>[3x]ATVGPRVIVVGAGMSGISAAKRLSEAGITDLLILEATDHIGGRMHKTNFAGINVELGANWVEGVNGGKMNPIWPIVN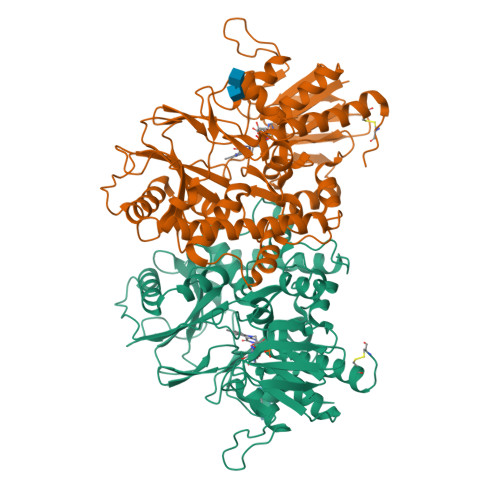STLKLRNFRSDFDYLAQNVYKEDGGVYDEDYVQKRIELADSVEEMGEKLSATLHASGRDDMSILAMQRLNEHQPNGPATPVDMVVDYYKFDYEFAEPPRVTSLQNTVPLATFSDFGDDVYFVADQRGYEAVVYYLAGQYLKTDDKSGKIVDPRLQLNKVVREIKYSPGGVTVKTEDNSVYSADYVMVSASLGVLQSDLIQFKPKLPTWKVRAIYQFDMAVYTKIFLKFPRKFWPEGKGREFFLYASSRRGYYGVWQEFEKQYPDANVLLVTVTDEESRRIEQQSDEQTKAEIMQVLRKMFPGKDVPDATDILVPRWWSDRFYKGTFSNWPVGVNRYEYDQLRAPVGRVYFTGEHTSEHYNGYVHGAYLSGIDSAEILINCAQKKMCKYHVQGKYD N-[2-{[benzyl(methyl)amino]methyl}-3-(4-fluoro-2-methoxyphenyl)-5-(propan-2-yl)-1H-indol-7-yl]methanesulfonamide 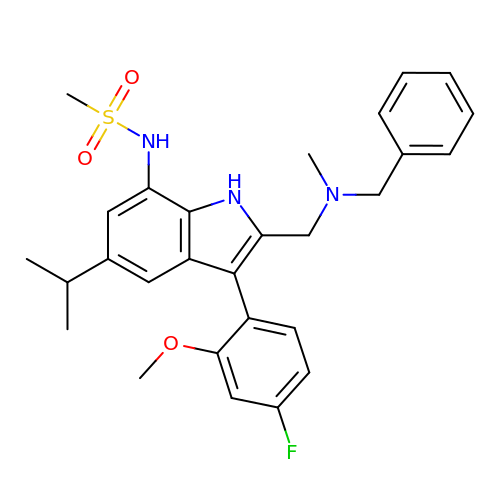| C28 H32 F N3 O3 S | MFAGIEMFDDDLMT-UHFFFAOYSA-N> MNVYDDVLDATVVSHSLATHFTTSDYEELLVVRTNILSVYRPTRDGKLYLTDEFKFHGLITDIGLIPQKDSPLSCLLLCTGVAKISILKFNTLTNSIDTLSLHYYEGKFKGKSLVELAKISTLRMDPGSSCALLFNNDIIAFLPFHVNKNDDDEEEEDEDENIDDSELIHSMNQKSQGTNTFNKRKRTKLGDKFTAPSVVLVASELYEGAKNIIDIQFLKNFTKPTIALLYQPKLVWAGNTTISKLPTQYVILTLNIQPAESATKIESTTIAFVKELPWDLHTIVPVSNGAIIVGTNELAFLDNTGVLQSTVLLNSFADKELQKTKIINNSSLEIMFREKNTTSIWIPSSKSKNGGSNNDETLLLMDLKSNIYYIQMEAEGRLLIKFDIFKLPIVNDLLKENSNPKCITRLNATNSNKNMDLFIGFGSGNALVLRLNNLKSTIETREAHNPSSGTNSLMDINDDDDEEMDDLYADEAPENGLTTNDSKGTVETVQPFDIELLSSLRNVGPITSLTVGKVSSIDDVVKGLPNPNKNEYSLVATSGNGSGSHLTVIQTSVQPEIELALKFISITQIWNLKIKGRDRYLITTDSTKSRSDIYESDNNFKLHKGGRLRRDATTVYISMFGEEKRIIQVTTNHLYLYDTHFRRLTTIKFDYEVIHVSVMDPYILVTVSRGDIKIFELEEKNKRKLLKVDLPEILNEMVITSGLILKSNMCNEFLIGLSKSQEEQLLFTFVTADNQIIFFTKDHNDRIFQLNGVDQLNESLYISTYQLGDEIVPDPSIKQVMINKLGHDNKEEYLTILTFGGEIYQYRKLPQRRSRFYRNVTRNDLAITGAPDNAYAKGVSSIERIMHYFPDYNGYSVIFVTGSVPYILIKEDDSTPKIFKFGNIPLVSVTPWSERSVMCVDDIK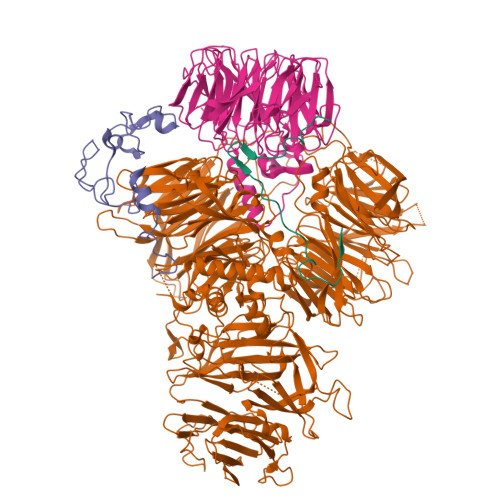NARVYTLTTDNMYYGNKLPLKQIKISNVLDDYKTLQKLVYHERAQLFLVSYCKRVPYEALGEDGEKVIGYDENVPHAEGFQSGILLINPKSWKVIDKIDFPKNSVVNEMRSSMIQINSKTKRKREYIIAGVANATTEDTPPTGAFHIYDVIEVVPEPGKPDTNYKLKEIFQEEVSGTVSTVCEVSGRFMISQSQKVLVRDIQEDNSVIPVAFLDIPVFVTDSKSFGNLLIIGDAMQGFQFIGFDAEPYRMISLGRSMSKFQTMSLEFLVNGGDMYFAATDADRNVHVLKYAPDEPNSLSGQRLVHCSSFTLHSTNSCMMLLPRNEEFGSPQVPSFQNVGGQVDGSVFKIVPLSEEKYRRLYVIQQQIIDRELQLGGLNPRMERLANDFYQMGHSMRPMLDFNVIRRFCGLAIDRRKSIAQKAGRHAHFEAWRDIINIEFSMRSLCQGK;> MSLIHPDTAKYPFKFEPFLRQEYSFSLDPDRPICEFYNSREGPKSCPRGPLCPKKHVLPIFQNKIVCRHWLRGLCKKNDQCEYLHEYNLRKMPECVFFSKNGYCTQSPDCQYLHIDPASKIPKCENYEMGFCPLGSSCPRRHIKKVFCQRYMTGFCPLGKDECDMEHPQFIIPDEGSKLRIKRDDEINTRKMDEEKERRLNAIINGEV;> MTYKYNCCDDGSGTTVGSVVRFDNVTLLIDPGWNPSKVSYEQCIKYWEKVIPEIDVIILSQPTIECLGAHSLLYYNFTSHFISRIQVYATLPVINLGRVSTIDSYASAGVIGPYDTNKLDLEDIEISFDHIVPLKYSQLVDLRSRYDGLTLLAYNAGVCPGGSIWCISTYSEKLVYAKRWNHTRDNILNAASILDATGKPLSTLMRPSAIITTLDRFGSSQPFKKRSKIFKDTLKKGLSSDGSVIIPVDMSGKFLDLFTQVHELLFESTKINAHTQVPVLILSYARGRTLTYAKSMLEWLSPSLLKTWENRNNTSPFEIGSRIKIIAPNELSKYPGSKICFVSEVGALINEVIIKVGNSEKTTLILTKPSFECASSLDKILEIVEQDERNWKTFPEDGKSFLCDNYISIDTIKEEPLSKEETEAFKVQLKEKKRDRNKKILLVKRESKKLANGNAIIDDTNGERAMRNQDILVENVNGVPPIDHIMGGDEDDDEEEENDNLLNLLKDNSEKSAAKKNTEVPVDIIIQPSAASKHKMFPFNPAKIKKDDYGTVVDFTMFLPDDSDNVNQNSRKRPLKDGAKTTSPVNEEDNKNEEEDGYNMSDPISKRSKHRASRYSGFSGTGEAENFDNLDYLKIDKTLSKRTISTVNVQLKCSVVILNLQSLVDQRSASIIWPSLKSRKIVLSAPKQIQNEEITAKLIKKNIEVVNMPLNKIVEFSTTI;> MDGHNQNQYQNQNQIQQSQQPPLKKYVTQRRSVDVSSPYINLYYNRRHGLPNLVVEPETSYTIDIMPPNAYRGRDRVINLPSKFTHLSSNKVKHVIPAIQWTPEGRRLVVATYSGEFSLWNASSFTFETLMQAHDSAVTTMKYSHDSDWMISGDADGMIKIWQPNFSMVKEIDAAHTESIRDMAFSSNDSKFVTCSDDNILKIWNFSNGKQERVLSGHHWDVKSCDWHPEMGLIASASKDNLVKLWDPRSGNCISSILKFKHTVLKTRFQPTKGNLLMAISKDKSCRVFDIRYSMKELMCVRDETDYMTLEWHPINESMFTLACYDGSLKHFDLLQNLNEPILTIPYAHDKCITSLSYNPVGHIFATAAKDRTIRFWTRARPIDPNAYDDPTYNNKKINGWFFGINNDINAVREKSEFGAAPPPPATLEPHALPNMNGFINKKPRQEIPGIDSNIKSSTLPGLSI>[2x]GSHGQYLLPEAKAQDSDKICVVIDLDETLVHSSFKPVNNADFIIPVEIDGVVHQVYVLKRPHVDEFLQRMGELFECVLFTASLAKYADPVADLLD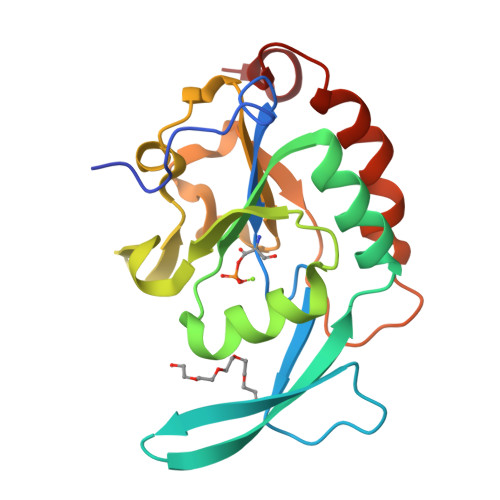KWGAFRARLFRESCVFHRGNYVKDLSRLGRDLRRVLILANSPASYVFHPDNAVPVASWFDNMSDTELHDLLPFFEQLSRVDDVYSVLRQ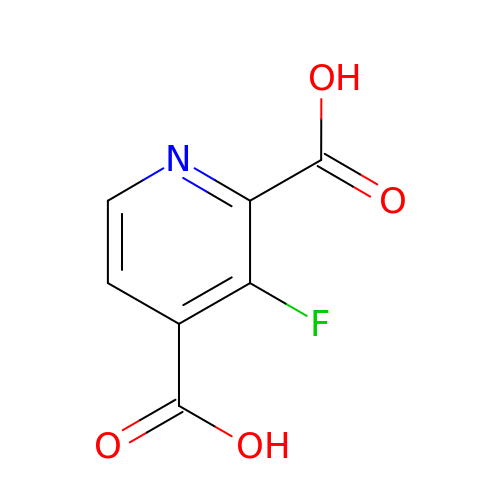3-fluoranylpyridine-2,4-dicarboxylic acid | C7 H4 F N O4 | IEQUQLPYQQVCNF-UHFFFAOYSA-N>[3x]ASNFTQFVLVDNGGTGDVTVAPSNFANGVAEWISSNSRSQAYKVTCSVRQSSAQNRKYTIKVEVPKVATQTVGGVELPVAAWRSYLN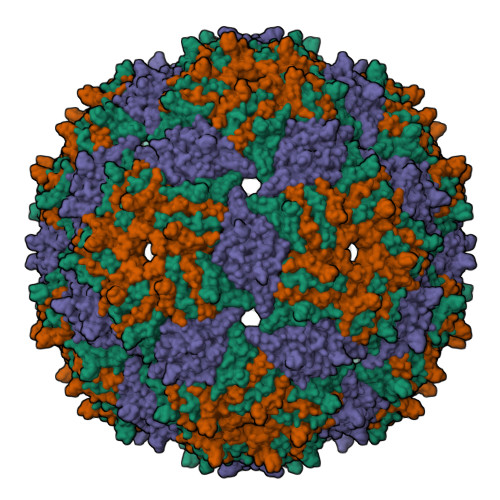MELTIPIFATNSDCELIVKAMQGLLKDGNPIPSAIAANSGIY>[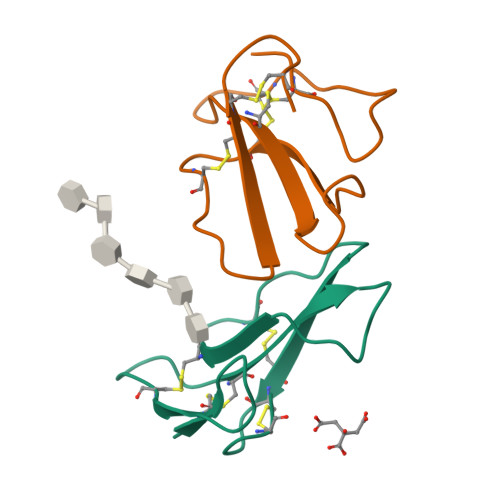2x]LKCNKLVPLFYKTCPAGKNLCYKMFMVATPKVPVKRGCIDVCPKSSLLVKYVCCNTDRCN> MDSRTKGKTVMEVGGDGVAVITLINPPVNSLSFDVLYNLKSNYEEALSRNDVKAIVITGAKGRFSGGFDISGFGEMQKGNVKEPKAGYISIDIITDLLEAARKPSVAAIDGLALGGGLELAMACHARISAPAAQLGLPELQLGVIPGFGGTQRLPRLVGLTKALEMILTSKPVKAEEGHSLGLIDAVVPPAELVTTARRWALDIVGRRKPWVSSVSKTDKLPPLGEAREILTFAKAQTLKRAPNMKHPLMCLDAIEVGIVSGPRAGLEKEAEVASQVVKLDTTKGLIHVFFSQRGTAKVPGVTDRGLVPRKIKKVAIIGGGLMGSGIATALILSNYPVILKEVNEKFLEAGIGRVKANLQSRVRKGSMSQEKFEKTMSLLKGSLDYESFRDVDMVIEAVIENISLKQQIFADLEKYCPQHCILASNTSTIDLNKIGERTKSQDRIVGAHFFSPAHIMPLLEIVRTNH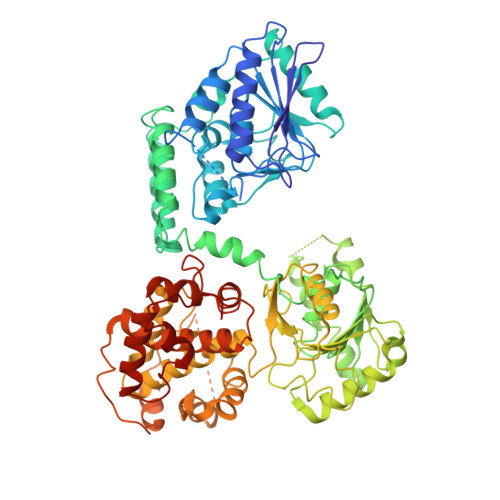TSAQVIVDLLDVGKKIKKTPVVVGNCTGFAVNRMFFPYTQAAMFLVECGADPYLIDRAISKFGMPMGPFRLCDLVGFGVAIATATQFIENFSERTYKSMIIPLMQEDKRAGEATRKGFYLYDDKRKAKPDPELKKYIEKARSISGVKLDPKLANLSEKDIIEMTFFPVVNEACRVFAEGIAVKAADLDIAGIMGMGFPPYRGGIMFWADSIGSKYIYSRLDEWSKAYGEFFKPCAFLAERGSKGVLLSAPVKQASSRL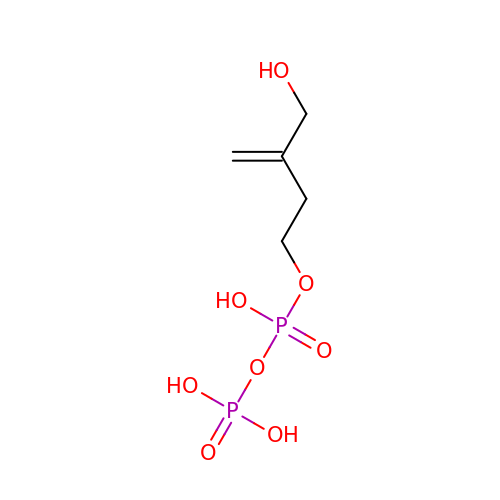3-(hydroxymethyl)but-3-en-1-yl trihydrogen diphosphate | C5 H12 O8 P2 | DFMXRQRICFHJAS-UHFFFAOYSA-N>[2x]MVVKFTKSEALHKEALEHIVGGVNSPSRSFKAVGGGAPIAMERGKGAYFWDVDGN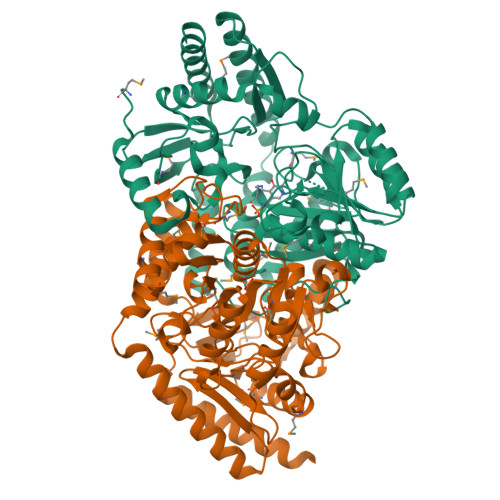KYIDYLAAYGPIITGHAHPHITKAITTAAENGVLYGTPTALEVKFAKMLKEAMPALDKVRFVNSGTEAVMTTIRVARAYTGRTKIMKFAGCYHGHSDLVLVAAGSGPSTLGTPDSAGVPQSIAQEVITVPFNNVETLKEALDKWGHEVAAILVEPIVGNFGIVEPKPGFLEKVNELVHEAGALVIYDEVITAFRFMYGGAQDLLGVTPDLTALGKVIGGGLPIGAYGGKKEIMEQVAPLGPAYQAGTMAGNPASMASGIACLEVLQQEGLYEKLDELGATLEKGILEQAAKHNIDITLNRLKGALTVYFTTNTIEDYDAAQDTDGEMFGKFFKLMLQEGVNLAPSKYEAWFLTTEHTKEDIEYTIEAVGRAFAALADNK>[4x]EAGITGTWYNQLGSTFIVTAGADGALTGTYESAVGNAESRYVLTGRYDSA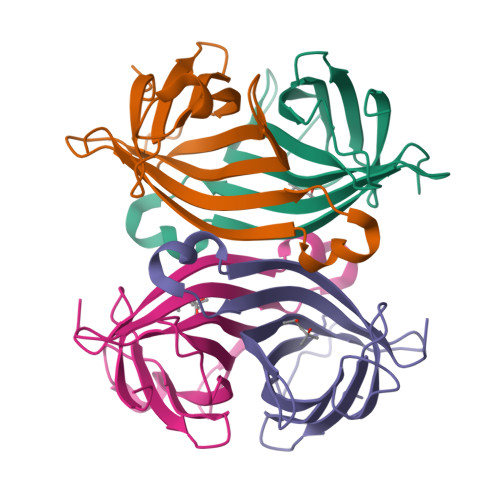PATDGSGTALGWTVAWKNNYRNAHSATTWSGQYVGGAEARINTQWLLTSGTTEANAWKSTLVGHDTFTKVKPS>MAHHHHHHMEPSVKESVSRIPLLKTKAGPRDGDKWTARLKEEYASLITYVEHNKASDSHWFHLESNPQGTRWYGTCWTYYKNEKYEFEMNFDIPVTYPQAPPEIALPELEGKTVKMYRGGKICMTTHFFPLW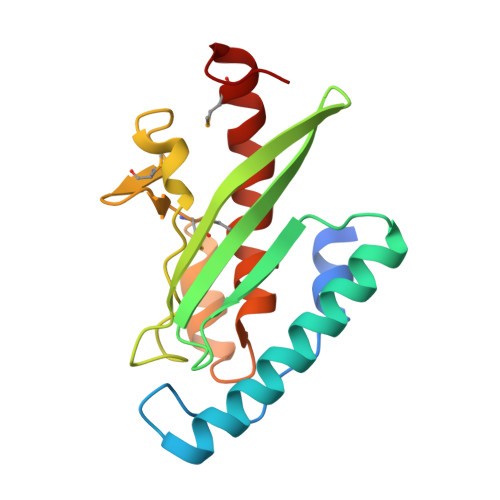ARNVPYFGISHVLALGLGPWLSIEVPAMVEEGYLKP[3x]> MNYLEGVGSKKGGGGIASESQFNLQRRKEVESLLSKGENVPYTFQDEKDDQVRSNPYIYKNHSGKLVCKLCNTMHMSWSSVERHLGGKKHGLNVLRRGISIEKSSLGREGQTTHDFRQQQKXXXXXXXXXXXXXXXXIIEAKQSLKNNGTIPVCKIATVKNPKNGSVGLAIQVNYSSEVKENSVDS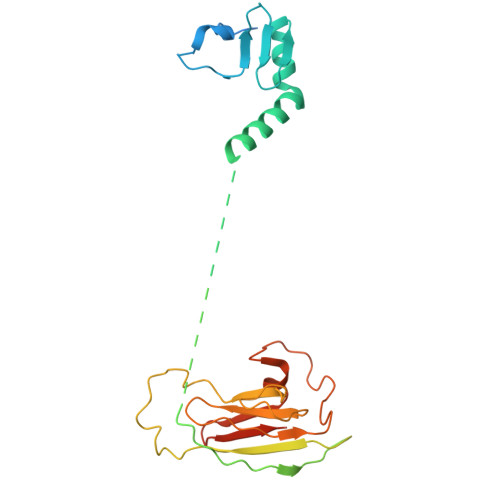DDKAKVPPLIRIVSGLELSDTKQKGKKFLVIAYEPFENIAIELPPNEILFSENNDMDNNNDGVDELNKKCTFWDAISKLYYVQFFFKQAEQEQADV methyl 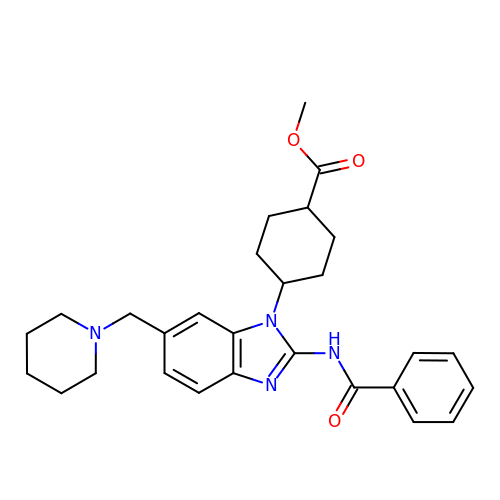cis-4-[2-(benzoylamino)-6-(piperidin-1-ylmethyl)-1H-benzimidazol-1-yl]cyclohexanecarboxylate | C28 H34 N4 O3 | NFTRTTWPZBZTLY-ZRZAMGCNSA-N>MELWLVRHGETLWNREGRLLGWTDLPLTAEGEAQARRLKGALPSLPAFSSDLLRARRTAELAGFSPRLYPELREIHFGALEGALWETMDPRYKEALLRFQGFHPPGGESLSAFQERVFRFLEGLKAPAVLFTHGGVVRAVLRALGEDGLVPPGSAVAVDWPRRVLVRLALDGEEATG[2x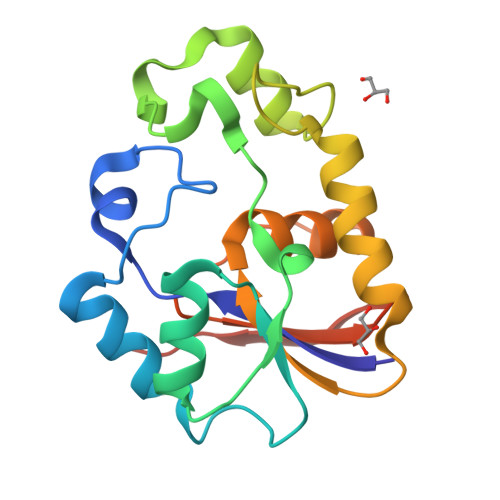]>[2x]VEGRFQLVAPYEPQGDQPQAIAKLVDGLRRGVKHQTLLGATGTGKTFTISNVIAQVNKPTLVIAHNKTLAGQLYSELKEFFPHNAVEYFVSYYDYYQPEAYVPQTDTYIEKDAKINDEIDKLRHSATSALFERRDVIIVASVSSIYGLGSPEEYRELVVSLRVGMEIERNALLRRLVDIQYDRNDIDFRRGTFRVRGDVVEIFPASRDEHSIRVEFFGDEIERIREVDALTGEVLGEREHVAIFPASHFVCREEKMRLAIQNIEQELEERLAELRAQGKLLEAQRLEQRTRYDLEMMREMGFSSGIENYSRHLALRPPGSTPYTLLDYFPDDFLIIVDESHVTLPQLRGMYNGDRARKQVLVDHGFRLPSALDNRPLTFEEFEQKINQIIYVSATPGPYELEHSPGVVEQIIRPTGLLDPTIDVRPTKGQIDDLIGEIRERVERNERTLVTTLTKKMAEDLTDYLKEAGIKVAYLHSEIKTLERIEIIRDLRLGKYDVL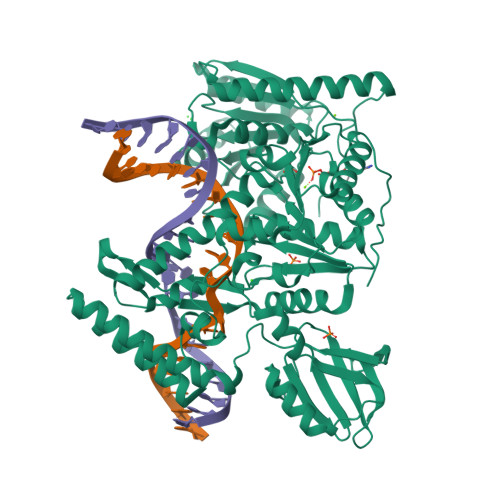VGINLLREGLDIPEVSLVAILDADKEGFLRSERSLIQTIGRAARNANGHVIMYADTITKSMEIAIQETKRRRAIQEEYNRKHGIVPRTVKKEIR> MSHHHHHHSQGGPQDHVEIIPLGGMGEIGKNITVFRFRDEIFVLDGGLAFPEEGMPGVDLLIPRVDYLIEHRHKIKAWVLTHGHEDHIGGLPFLLPMIFGKESPVPIYGARLTLGLLRGKLEEFGLRPGAFNLKEISPDDRIQVGRYFTLDLFRMTHSIPDNSGVVIRTPIGTIVHTGDFKLDPTPIDGKVSHLAKVAQAGAEGVLLLIADATNAERPGYTPSEMEIAKELDRVIGRAPGRVFVTTFASHIHRIQSVIWAAEKYGRKVAMEGRSMLKFSRIALELGYLKVKDRLYTLEEVKDLPDHQVLILATGSQGQPMSVLHRLAFEGHAKMAIKPGDTVILSSSPIPGNEEAVNRVINRLYALGAYVLYPPTYKVHASGHASQEELKLILNLTTPRFFLPWHGEVRHQMNFKWLAESMSRPPEKTLIGENGAVYRLTRETFEKVGEVPHGVLYVDGLGVGDITEEILA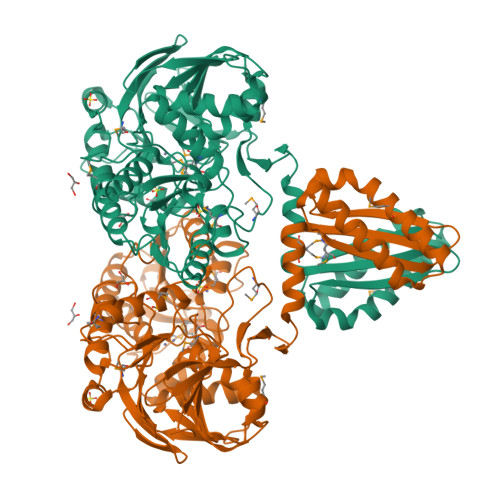DRRHMAEEGLVVITALAGEDPVVEVVSRGFVKAGERLLGEVRRMALEALKNGVREKKPLERIRDDIYYPVKKFLKKATGRDPMILPVVIEG> MKSNNKEESTKEDNKKEVVTVEHAMGKTEVPANPKRVVILTNEGTEALLELGVKPVGAVKSWTGDPWYPHIKDKMKDVKVVGDEGQVNVETIASLKPDLIIGNKMRHEKVYEQLKAIAPTVFSETLRGEWKDNFKFYAKALNKEKEGQKVVADYESRMKDLKGKLGDKVNQEISMVRFMPGDVRIYHGDTFSGVILKELGFKRPGDQNKDDFAERNVSKERISAMDGDVLFYFTF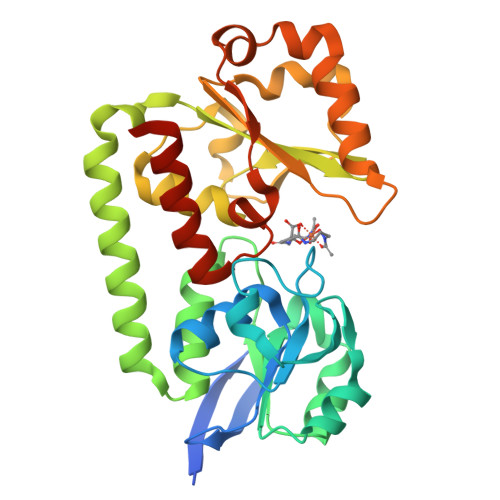DKGNEKKGSELEKEYINDPLFKNLNAVKNGKAYKVDDVIWNTAGGVIAANLLLDDIEKRFVKHHHHHH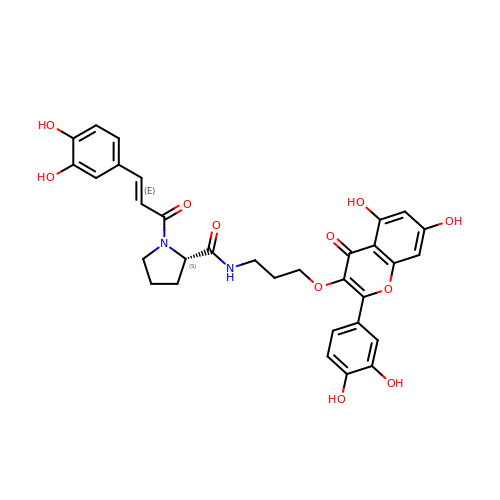N-(3-{[2-(3,4-dihydroxyphenyl)-5,7-dihydroxy-4-oxo-4H-1-benzopyran-3-yl]oxy}propyl)-1-[(2E)-3-(3,4-dihydroxyphenyl)prop-2-enoyl]-L-prolinamide | C32 H30 N2 O11 | MYJPTGWVMBCTRI-MRSBXDGLSA-N> KQGPTSVAYVEVNNNSMLNVGKYTLADGGGNAFDVAVIFAANINYDTGTKTAYLHFNENVQRVLDNAVTQIRPLQQQGIKVLLSVLGNHQGAGFANFPSQQAASAFAKQLSDAVAKYGLDGVDFADEYAEYGNNGTAQPNDSSFVHLVTALRANMPDKIISLYNIGPAASRLSYGGVDVSDKFDYAWNPYYGTWQVPGIALPKAQLSPAAVEIGRTSRSTVADLARRTVDEGYGVYLTY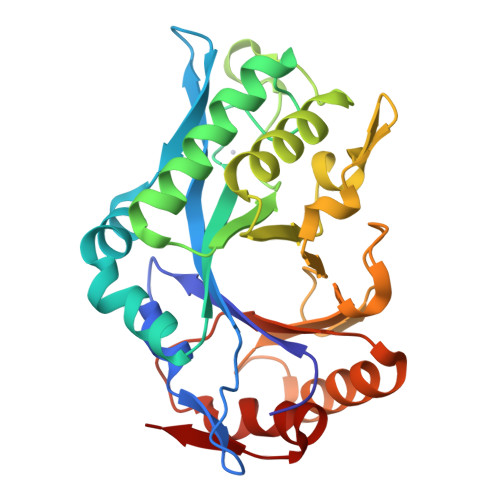NLDGGDRTADVSAFTRELYGSEAVRT>[2x]SSDEEFKFLATEAKMLITAAERLAGTDPELQEMVALIKKELEQA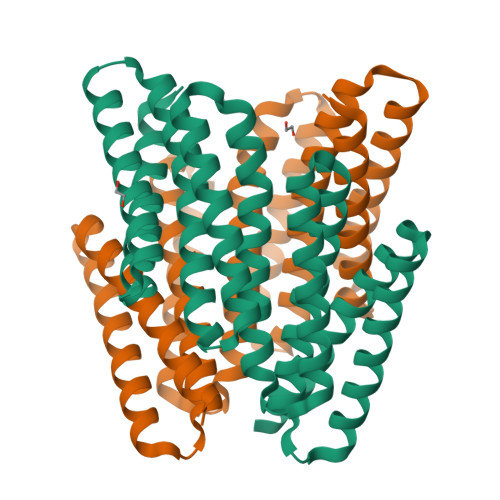ERTFRNGDKSEAQRQLEFVLTAARAVMNVAAAANAAGTDPELIEMVLRILKQLKEAIRTFQNGDQEEAETQLRFVLRAAIAVAVVAAALVLAGTDPELQEMVKQILEELKQAIETFARGDKEKALTQLLFVAWAAHAVAMIAAAANLAGTDPRLQQQVKEILEKLKEAIETFQKGDEEQAFRQLAEVLAEAALVALRAALTN1-(3,4-DICHLOROBENZYL)-7-PHENYL-1H-BENZIMIDAZOL-2-AMINE | C20 H15 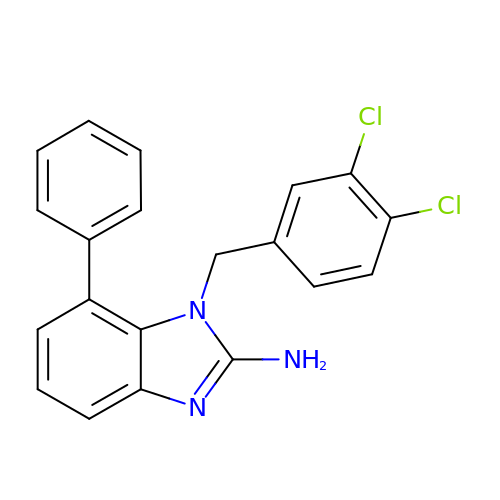Cl2 N3 | JFVMZMBFRZPOFF-UHFFFAOYSA-N>PGSVAENNLCSQYEEKVRPCIDLIDSLRALGVEQDLALPAIAVIGDQSSGKSSVLEALSGVALPRGSGIVTRCPLVLKLKKLVNEDKWRGKVSYQDYEIEISDASEVEKEINKAQNAIAGEGMGISHELITLEISSRDVPDLTLIDLPGITRVAVGNQPADIGYKIKTLIKKYIQRQETISLVVVPSNVDIATTEALSMAQEVDPEGDRTIGILTKPDLVD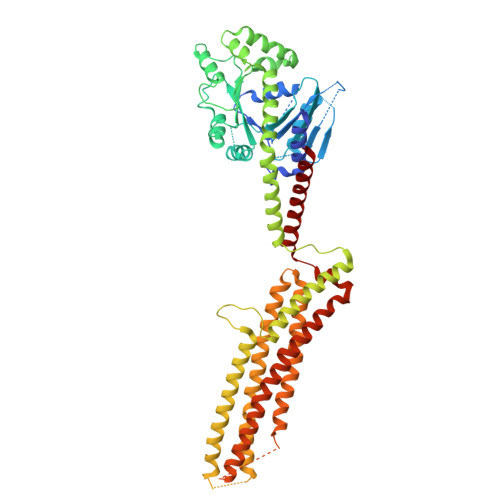KGTEDKVVDVVRNLVFHLKKGYMIVKCRGQQEIQDQLSLSEALQREKIFFENHPYFRDLLEEGKATVPCLAEKLTSELITHICKSLPLLENQIKETHQRITEELQKYGVDIPEDENEKMFFLSDKINAFNQDITALMQGEETVGEEDIRLFTRLRHEFHKWSTIIENNFQEGHKILSRKIQKFENQAAAAELPGFVNYRTFETIVKQQIKALEEPAVDMLHTVTDMVRLAFTDVSIKNFEEFFNLHRTAKSKIEDIRAEQEREGEKLIRLHFQDEQIVYGAFQSSSATDSSMEEIFQHLMAYHQEASKRISSHIPLIIQFFMLQTYGQQLQSAMSQLSQDKDTYSWLLKERSDTSDKRKFLKERLARLTQARRRLAQFPG[2x]>MTSITPVTLANCEDEPIHVPGAIQPHGALVTLRADGMVLAASENIQALLGFVASPGSYLTQEQVGPEVLRMLEEGLTGNGPWSNSVETRIGEHLFDVIGHSYKEVFYLEFEIRTADTLSITSFTLNAQRIIAQVQLHNDTASLLSNVTDELRRMTGYDRVMAYRFRHDDSGEVVAESRREDLESYLGQRYPASDIPAQARRLYIQNPIRLIADVAYTPMRVFPALNPETNESFDLSYSVLRSVSPIHCEYLTNMGVRASMSISIVVGGKLWGLFSCHHMSPKLIPYPVRMSFQIFSQVCSAIVERLEQGRIAELLRVSTERRLALARRARDADDLFGALAHPDDGIAALIPCDGALVMLGGRTLSIRGDFERQAGNVLQRLQRDPERDIYHTDNWPQPSEDSPDGGDCCGVLAIRFHR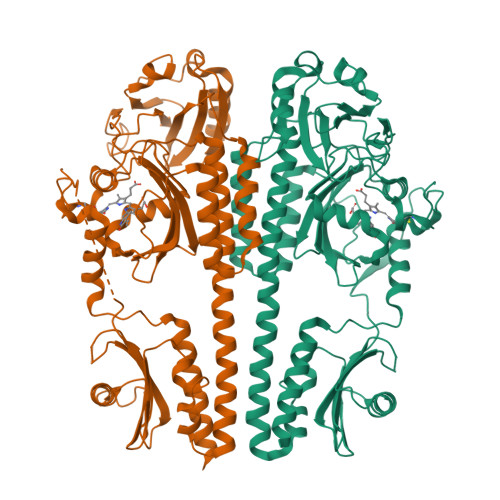QESGWIFWFRHEEVHRIRWGGKPEKLLTIGPSGPRLTPRGSFEAWEEVVRGHSTPWSETDLAIAEKLRLDLMELCLNHALEHHHHHH[8x]> RERPHTSGHHGAGEARATAPSTVSPYGPEARAELSSRLTTLRNTLAPATNDPRYLQACGGEKLNRFRDIQCRRQTAVRADLNANYIQVGNTRTIACQYPLQSQLESHFRMLAENRTPVLAVLASSSEIANQRFGMPDYFRQSGTYGSITVESKMTQQVGLGDGIMADMYTLTIREAGQKTISVPVVHVGNWPDQTAVSSEVTKALASLVDQTAETKRNMYESKGSSAVADDSKLRPVIHCR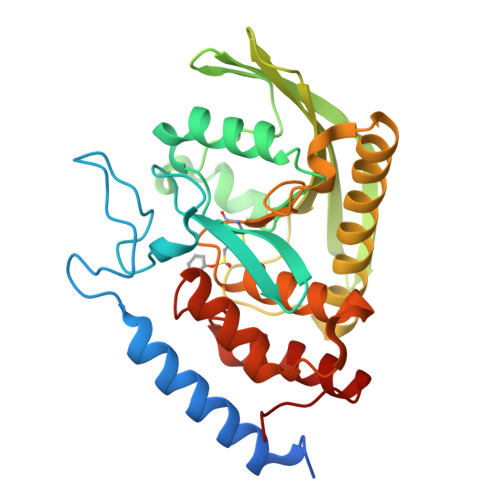AGVGRTAQLIGAMCMNDSRNSQLSVEDMVSQMRVQRNGIMVQKDEQLDVLIKLAEGQGRPLLNS> MKMLNKLAGYLLPIMVLLNVAPCLGQVVASNETLYQVVKEVKPGGLVQIADGTYKDVQLIVSNSGKSGLPITIKALNPGKVFFTGDAKVELRGEHLILEGIWFKDGNRAIQAWKSHGPGLVAIYGSYNRITACVFDCFDEANSAYITTSLTEDGKVPQHCRIDHCSFTDKITFDQVINLNNTARAIKDGSVGGPGMYHRVDHCFFSNPQKPGNAGGGIRIGYYRNDIGRCLVDSNLFMRQDSEAEIITSKSQENVYYGNTYLNCQGTMNFRHGDHQVAINNFYIGNDQRFGYGGMFVWGSRHVIACNYFELSETIKSRGNAALYLN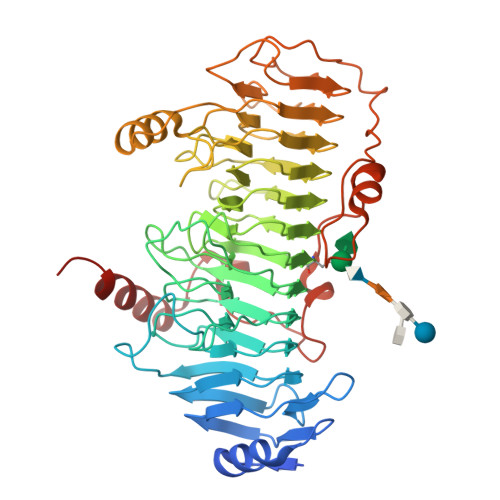PGAMASEHALAFDMLIANNAFINVNGYAIHFNPLDERRKEYCAANRLKFETPHQLMLKGNLFFKDKPYVYPFFKDDYFIAGKNSWTGNVALGVEKGIPVNISANRSAYKPVKIKDIQPIEGIALDLNALISKGITGKPLSWDEVRPYWLKEMPGTYALTARLSADRAAKFKAVIKRNKEH>[2x]GPGSMALERTLSIIKPDAVAKNVIGQIYSRFENAGLKIVAARMAHLSRADAEKFYAVHAERPFFKDLVEFMISGP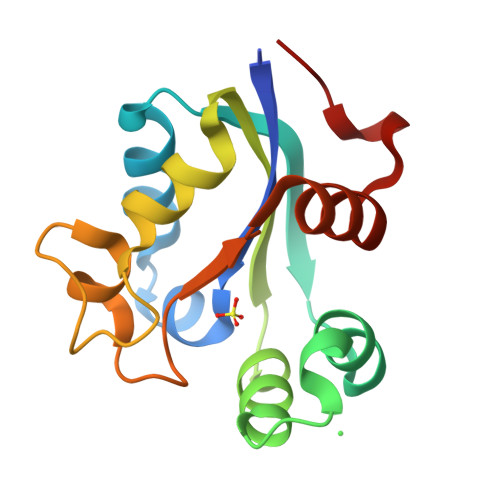VMIQVLEGEDAILKNRDLMGATDPKKAEKGTIRADFADSIDANAVHGSDAPETARVEIAFFFPEMNVYSR> PPPP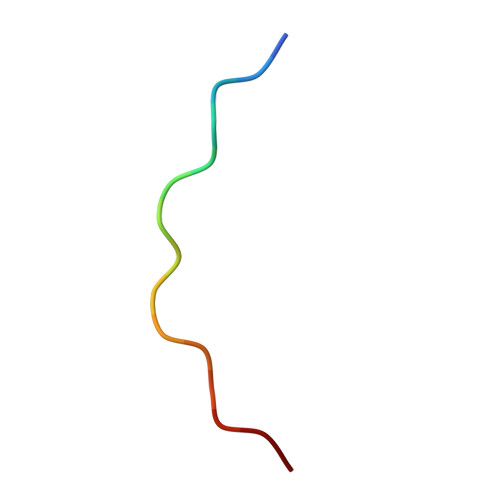PPPPPPPPPPP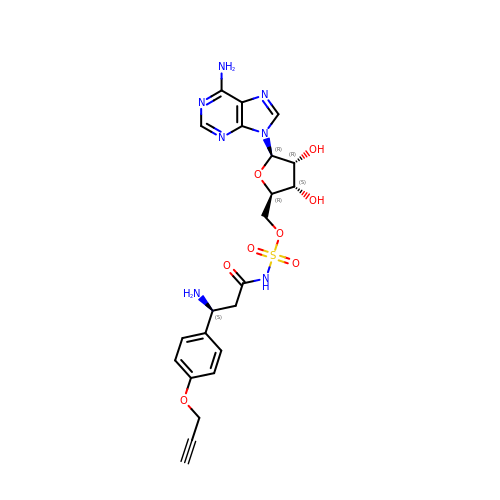[(2~{R},3~{S},4~{R},5~{R})-5-(6-aminopurin-9-yl)-3,4-bis(oxidanyl)oxolan-2-yl]methyl ~{N}-[(3~{S})-3-azanyl-3-(4-prop-2-ynoxyphenyl)propanoyl]sulfamate | C22 H25 N7 O8 S | SOQSTTVKSPLYCJ-KSHOWADASA-N> MKERFLERFSESAFLLERLTGIDGKILLAQSALETGWGRHTVGNNLFGIKKLSWLEGGVRAETKEFDGVKTIDTFQSFVSPENSMIAYLILIKECYNRAWECRKEPEKYF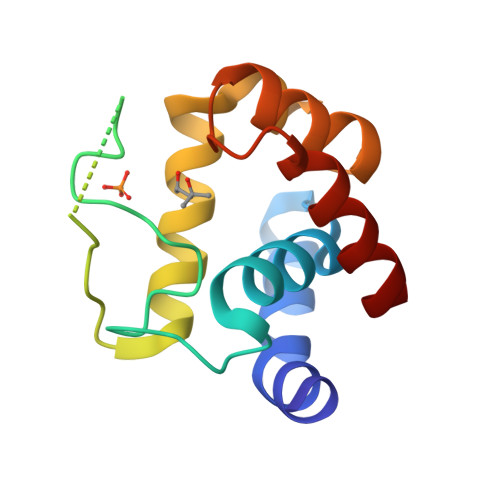RLLQRYGYATDPMYAEKCLDVYNCVE> GNYMGNPWTEYMAKYDIEEVHGSGIRVDLGEDAEVAGTQYRLPSGKCPVFGKGIIIENSNTTFLKPVATGNQDLKDGGFAFPPTNPLISPMTLNGMRDFYKNNEYVKNLDELTLCSRHAGNMNPDNDKNSNYKYPAVYDYNDKKCHILYIAAQENNGPRYCNKDQSKRNSMFCFRPAKDKLFENYTYLSKNVVDNWEEVCPRKNLENAKFGLWVDGNCEDIPHVNEFSANDLFECNKLVFELSASDQPKQYEQHLTDYEKIKEGFKNKNASMIKSAFLPTGAFKADRYKSHGKGYNWGNYNRETQKCEIFNVKPTCLINNSSYIATTA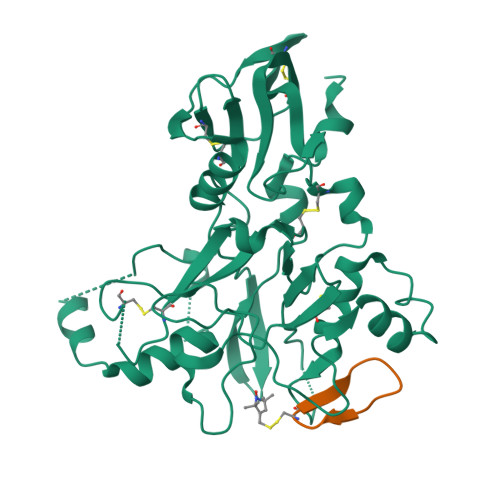LSHPIEVE;> CWTTRMSPPMQIP> MIAYYLIIAFLGISVTFNMLGSIALHRFPDVYTRLHGATKCTTFGTIFAALAVITHAIVKLQATGNPKYLQMAIHSFVAMLALLLTNPVGAH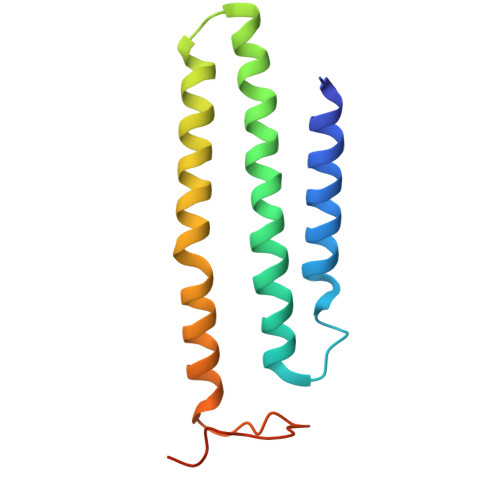AIAKAAHKTGYLPKRAVVDAYLEKERGEKNES methyl (4-{4-chloro-2-[(1S)-1-({(2E)-3-[5-chloro-2-(1H-tetrazol-1-yl)phenyl]prop-2-enoyl}amino)-2-phenylethyl]-1H-imidazol-5-yl}phenyl)carbamate 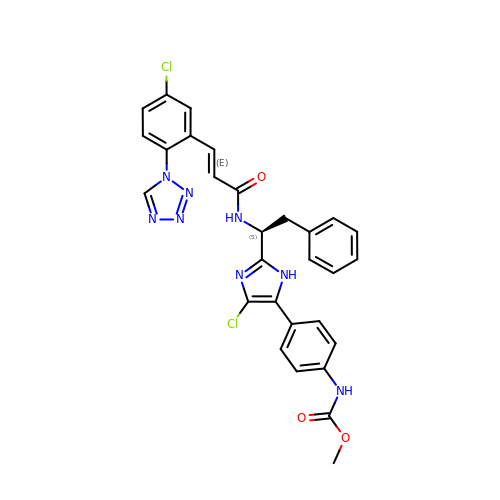| C29 H24 Cl2 N8 O3 | GLCBWRQIUCCILC-PZVJUEDKSA-N>[2x]MDSDTLSGLLENVAKKFPDRRALSVSGKFNLTHARLHDLIERAASRLVSDAGIKPGDVVALTFPNTVEFVIMFLAVIRARATAAPLNAAYTAEEFEFYLSDSDSKLLLTSKEGNAPAQEAASKLKISHVTATLLDAGSDLVLSVADSDSVVDSATELVNHPDDGALFLHTSGTTSRPKGVPLTQLNLASSVKNIKAVYKLTESDSTVIVLPLFHVHGLLAGLLSSLGAGAAVTLPAAGRFSATTFWPDMKKYNATWYTAVPTIHQIILDRHASHPETEYPKLRFIRSCSASLAPVILSRLEEAFGAPVLEAYAMTEATHLMSSNPLPEEGPHKPGSVGKPVGQEMAILNEKGEIQEPNNKGEVCIRGPNVTKGYKNNPEANKAGFEFGWFHTGDIGYFDTDGYLHLVGRIKELIN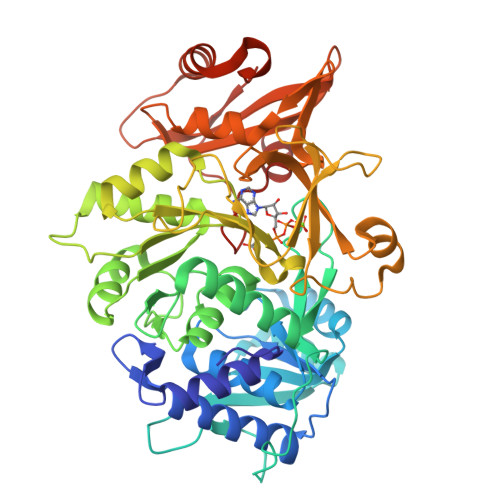RGGEKISPIEVDAVLLTHPDVSQGVAFGVPDEKYGEEINCAVIPREGTTVTEEDIKAFCKKNLAAFKVPKRVFITDNLPKTASGKIQRRIVAQHFLEKP> 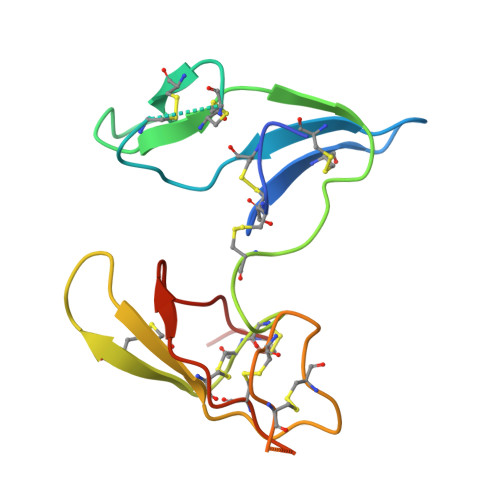AGKKRPWKCCDEAVCTRSIPPICTCMDEVFECPKTCKSCGPSMGDPSRRICQDQYVGDPGPICRPWECCDKAICTRSNPPTCRCVDEVKKCAPTCKTCLPSRSRPSRRVCIDSYFGPVPPRCTPR3-tert-butyl-N-[(5R)-2-{2-[3,5-dimethyl-1-(propan-2-yl)-1H-pyrazol-4-yl]-3H-imidazo[4,5-b]pyridin-7-yl}-6,7,8,9-tetrahydro-5H-benzo[7]annulen-5-yl]-1,2,4-oxadiazole-5-carboxamide 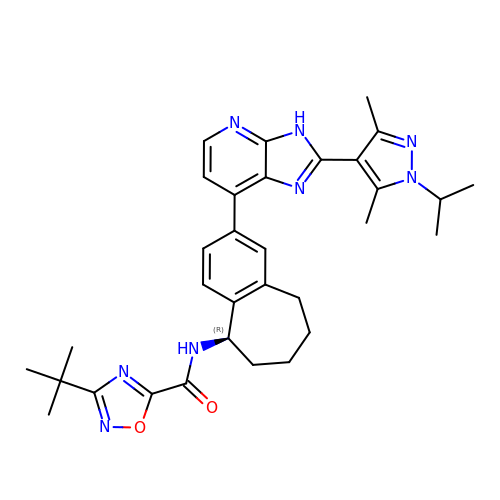| C32 H38 N8 O2 | XHKFYFCKCXKVPO-XMMPIXPASA-N>[2x]MVTLAELASDIQSQVKVIDTYLTEHNLPQPTFAPDSPRELPLDANVQRARLLLIEKAMALSNLAIGAADNLRWHCMNNKFDDMTLHFLARYNIFDAVPRDEPISYAELSKKVGLAEHRLRRIMSMAYTQHYFCTPKPGFVAHTSNSAMAIGDPLALAWI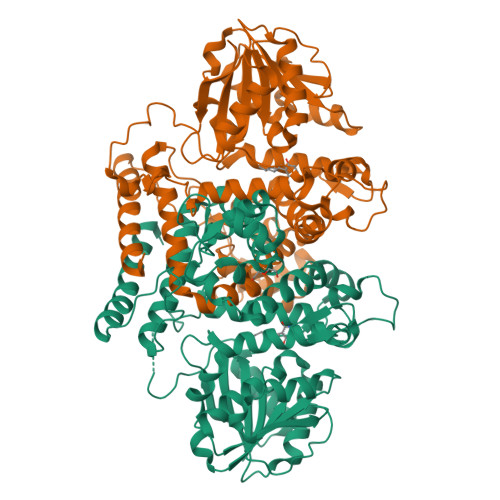LHNIEEVQPWYSNKLVDATMKWGDSIDPKHTGPNLNAKPGEEKLFYEIMEEDDQGEWNGVKGKGFRLWRLYDTDKFFGTGGAIKGTNLLRAFDWGGLGKATVVDIGGITGHLASTVALANPDLTFIVQERNQPWYEKQFYEQLPAELNGRVSYMPHDKYAEQPVKGADVYFMSTVLHKEPDDKAITILRRCVEAMDPNKSRLLTRDIVMDGGDPPAEDAVINGRAINSKEGSYEAGLGPTGVITRLNIGIDFQVLAVVNGFERTREEWVTLFKKADPRFALKGCIQTVGNCAALMEWILEE> SMAPPSTREPRVLSATSATKSDGEMVLPGFPDADSFVKFALGSVVAVTKASGGLPQFGDEYDFYRSFPGFQAFCETQGDRLLQCMSRVMQYHGCRSNIKDRSKVTELEDK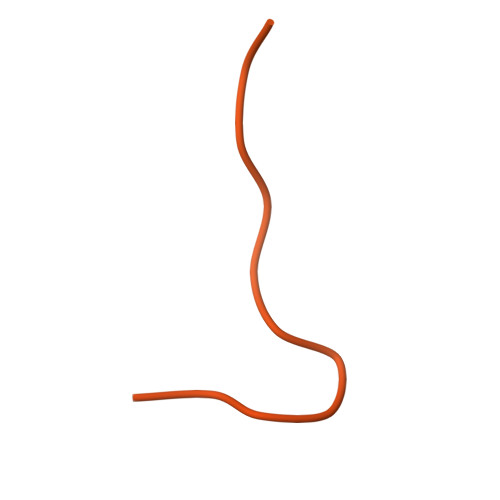FDLLVDANDVILERVGILLDEASGVNKNQQPVLPAGLQVPKTVVSSWNRKAAEYGKKAKSETFRLLHAKNIIRPQLKFREKIDNSNTPFLPKIFIKPNAQKPLPQALSKERRERPQDRPEDLDVPPALADFIHQQRTQQVEQDMFAHPYQYELNHFTPADAVLQKPQPQLYRPIEETPCHFISSLDELVELNEKLLNCQEFAVNLEHHSYRSFLGLTCLMQISTRTEDFIIDTLELRSDMYILNESLTDPAIVKVFHGADSDIEWLQKDFGLYVVNMFDTHQAARLLNLGRHSLDHLLKLYCNVDSNKQYQLADWRIRPLPEEMLSYARDDTHYLLYIYDKMRLEMWERGNGQPVQLQVVWQRSRDICLKKFIKPIFTDESYLELYRKQKKHLNTQQLTAFQLLFAWRDKTARREDESYGYVLPNHMMLKIAEELPKEPQGIIACCNPVPPLVRQQINEMHLLIQQAREMPLLKSEVAAGVKKSGPLPSAERLENVLFGPHDCSHAPPDGYPIIPTSGSVPVQKQASLFPDEKEDNLLGSRGSGSGSGSGSVSQAAKFDPSTKIYEISNRWKLAQVQVQKDSKEAVKKKAAEQTAAREQAKEACKAAAEQAISVRQQVVLENAAKKRERATSDPRTTEQKQEKKRLKISKK>[8x]GHMASGLTIYFKKPDSWGTPHLYYY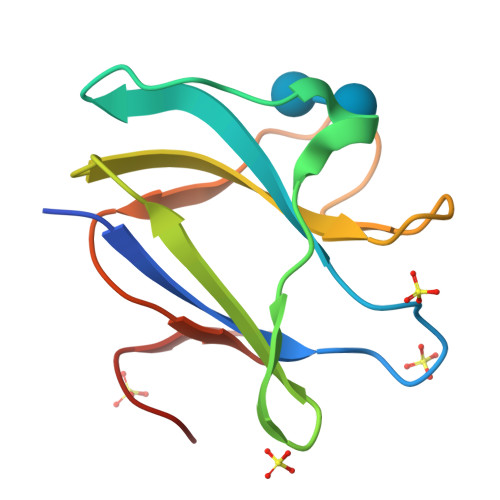DTNPKVDEPTWSEAPEMEHYEGDWYTHTIEGVESVRLLFKDRGTNQWPGPGEPGFFRDQDGWFDGEWHVDRPG>[2x]GPGYQDPLTINADLQRVAEESLNAAVKRVGGVWGSAAVLEIGTGRLLALAPGGTRSVSAIYEPGSVGKLV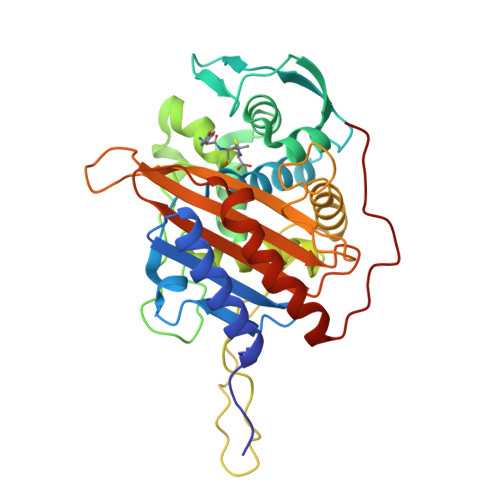TLAAAIDQKKVTPTSTFTVSSTRDMPNGERISDDSPHETQDMTVAGIIAHSYNTGTVQIGDTVSDSVRYEYMQKFGWGAKTGITLPSEESGILRPHTEWGDRDHYTTMFGQGVAVTTIQLAQMVAVFGQKGVLIPPRIIDGYDDENGVYTPTVMGESRQVVSEDTAQTVLNIMQGATQPGGTAEGIGAVKGYNVAAKTGTAENVGSSGSLTDTAATFTALIPAENPKIAVAVVIYKENGTVYGSTASAPVFVDIAQFAMREMKIPPSTVPLYKYPW>[4x]MSLARVLLNIHGTGDTVVLALCDEDLLGVELKYKGRTLHISEPFYSGKSMEPDRAAKKIREAVQ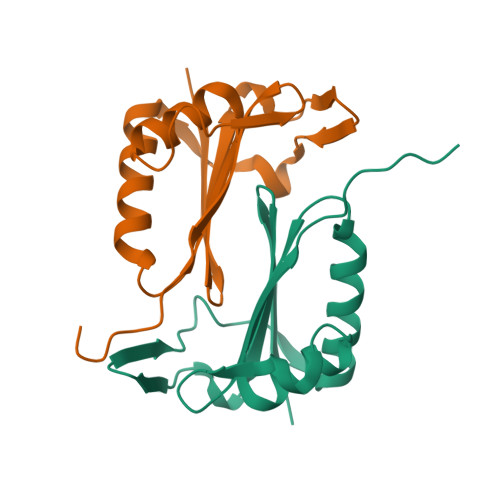EYEDEKTVAINALGELACSVVVDAGLAREDEIGELGGVPHVQMYILPREPFLEGHHHHHH>[2x]GSVISDFIYQGASLHNQTDRTGETALHLAARYSRSDAAKRLLEASADANIQDNMGRTPLHAAVSADAQGVFQILLRNRATDLDARMHDGTTPLILAAR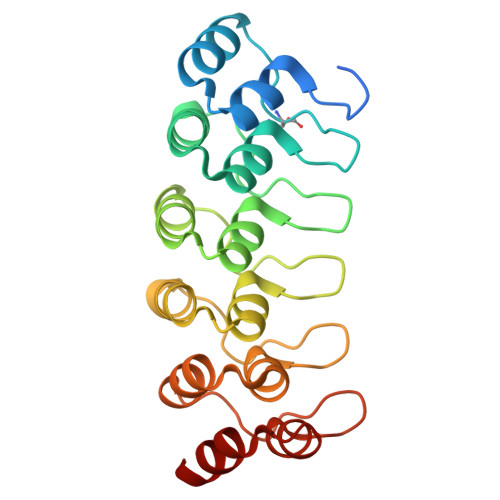LALEGMLEDLINSHADVNAVDDLGKSALHWAAAVNNVDAAVVLLKNGANKDMQNNKEETPLFLAAREGSYETAKVLLDHFANRDITDHMDRLPRDIAQERMHHDIVRLLDEY>[4x]GMSVGEAMDTEVRAAAQAVCLAFNENPEAVEPRVQAAIAAAAARINRYPFDAEPRVMRKLAEHFSCPEDNLMLVRGIDECFDRISAEFSSMRFVTAWPGFDGYRARIAVSGLRHFEIGLTDDLLLDPNDLAQVSRDDCVVLANPSNP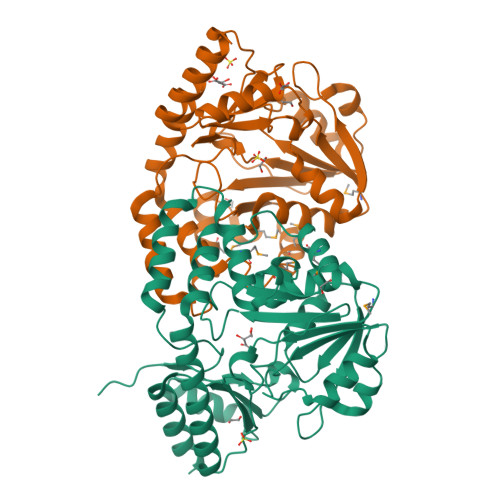TGQALSAGELDQLRQRAGKLLIDETYVDYSSFRARGLAYGENELVFRSFSKSYGLAGLRLGALFGPSELIAAMKRKQWFCNVGTLDLHALEAALDNDRAREAHIAKTLAQRRRVADALRGLGYRVASSEANFVLVENAAGERTLRFLRERGIQVKDAGQFGLHHHIRISIGREEDNDRLLAALAEYSDHS> GGUCAAAUAGGUGCCGG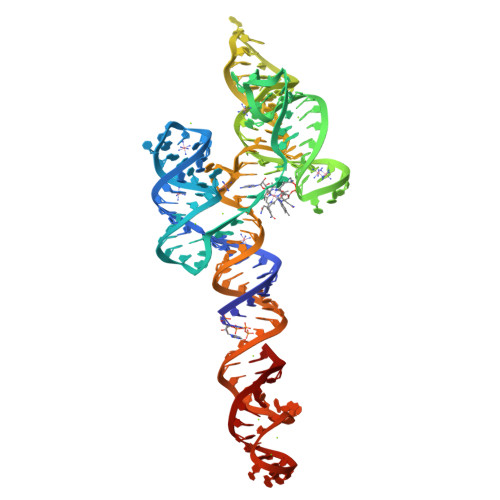UCCGUGAACAACAGCCGGCUUAAAAGGGAAACCGGUAAAAGCCGGUGCGGUCCCGCCACUGUAAUUGGCCAAGCGCCAAGAGCCAGGAUACCUGCCUGUUUGAUCAGCACGAAUUCUGCGAGGACAGAUGA>MNFYSAYQHGFVRVAACTHHTTIGDPAANAASVLDMARACHDDGAALAVFPELTLSGYSIEDVLLQDSLLDAVEDALLDLVTESADLLPVLVVGAPLRHRHRIYNTAVVIHRGAVLGVVPKSYLPTYREFYERRQMAPGDGERGTIRIGGADVAFGTDLLFAASDLPGFVLHVEIAEDMFVPMPPSAEAALAGATVLANLSGSPITIGRAEDRRLLARSASARCLAAYVYAAAGEGESTTDLAWDGQTMIWENGALLAESERFPKGVRRSVADVDTELLRSERLRMGTFDDNRRHHRELTESFRRIDFALDPPAGDIGLLREVERFPFVPADPQRLQQDCYEAYNIQV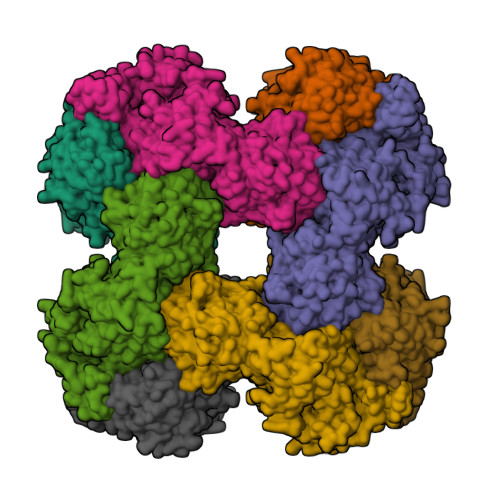SGLEQRLRALDYPKVVIGVSGGLDSTHALIVATHAMDREGRPRSDILAFALPGFATGEHTKNNAIKLARALGVTFSEIDIGDTARLMLHTIGHPYSVGEKVYDVTFENVQAGLRTDYLFRIANQRGGIVLGTGDLSELALGWSTYGVGDQMSHYNVNAGVPKTLIQHLIRWVISAGEFGEKVGEVLQSVLDTEITPELIPTGEEELQSSEAKVGPFALQDFSLFQVLRYGFRPSKIAFLAWHAWNDAERGNWPPGFPKSERPSYSLAEIRHWLQIFVQRFYSFSQFKRSALPNGPKVSHGGALSPRGDWRAPSDMSARIWLDQIDREVPKG[4x]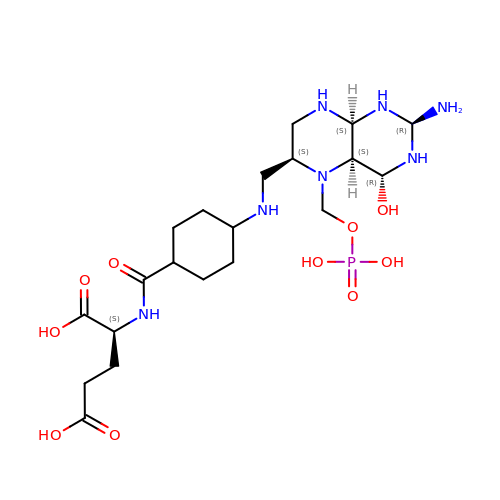N-({trans-4-[({(2R,4R,4aS,6S,8aS)-2-amino-4-hydroxy-5-[(phosphonooxy)methyl]decahydropteridin-6-yl}methyl)amino]cyclohexyl}carbonyl)-L-glutamic acid | C20 H38 N7 O10 P | YEQBTMZGNSUQID-NLSVEUOSSA-N> SMDATPNAVELTVDNAWFIAETIGAGTFPWVLAITMPYSDAAQRGAFVDRQRDELTRMGLLSPQGVINPAVADWIKVVCFPDRWLDL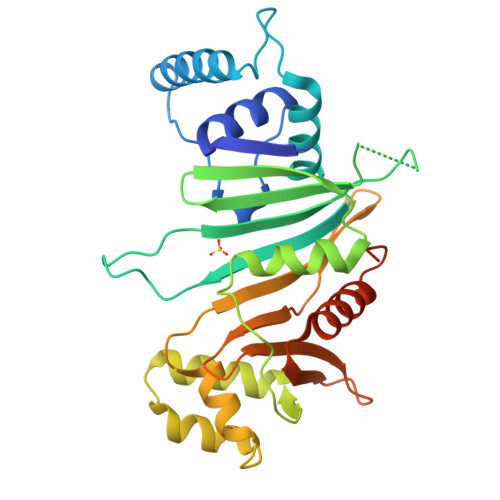RYVGPASADGACELLRGIVALRTGTGKTSNKTGNGVVALRNAQLVTFTAMDIDDPRALVPILGVGLAHRPPARFDEFSLPTRVGARADERLRSGVPLGEVVDYLGIPASARPVVESVFSGPRSYVEIVAGCNRDGRHTTTEVGLSIVDTSAGRVLVSPSRAFDGEWVSTFSPGTPFAIAVAIQTLTACLPDGQWFPGQRVSRDFSTQSS> MKFTVEREHLLKPLQQVSGPLGGRPTLPILGNLLLQVADGTLSLTGTDLEMEMVARVALVQPHEPGATTVPARKFFDICRGLPEGAEIAVQLEGERMLVRSGRSRFSLSTLPAADFPNLDDWQSEVEFTLPQATMKRLIEATQFSMAHQDVRYYLNGMLFETEGEELRTVATDGHRLAVCSMPIGQSLPSHSVIVPRKGVIELMRMLDGGDNPLRVQIGSNNIRAHVGDFIFTSKLVDGRFPDYRRVLPKNPDKHLEAGCDLLKQAFARAAAASNEKFRGVRLYVSENQLKITANNPEQEEAEEILDVTYSGAEMEIGFNVSYVLDVLNALKCENVRMMLTDSVSSVQIEDAASQSAAYVVMPMR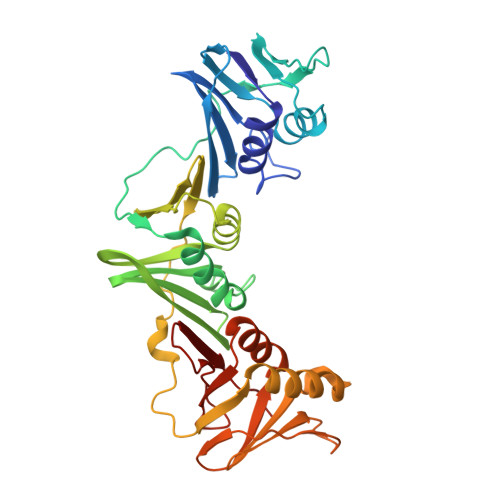L>SPNIKIFSGSSHQDLSQKIADRLGLELGKVVTKKFSNQETCVEIGESVRGEDVYIVQSGCGEINDNLMELLIMINACKIASASRVTAVIPCFPYARQDKKDKVGESRAPISAKLVANMLSVAGADHIITMDLHASQIQGFFDIPVDNLYAEPAVLKWIRENISEWRNCTIVSPDAGGAKRVTSIADRLNVDFALIHKERKKANEVDRMVLVGDVKDRVAILVDDMADTCGTICHAADKLLSAGATRVYAILTHGIFSGPAISRINNACFEAVVVTNTIPQEDKMKHCSKIQVIDISMILAEAIRRTHNGESVSYLFSHVPL[18x]

Phosphoribosyl pyrophosphate synthetase (PRPS) stands as the first and rate-limiting enzyme in the purine biosynthesis pathway. It catalyzes the pyrophosphorylation of D-ribose-5-phosphate (R5P), obtained from the glucose pentose phosphate pathway (PPP), at the 1’ hydroxyl group position, yielding the catalytic product 5-phosphoribosyl-ɑ-1-pyrophosphate (PRPP). PRPP serves as an essential metabolic intermediate for purine biosynthesis via both de novo and salvage pathways, as well as for the synthesis of pyrimidines, amino acids (tryptophan and histidine), and co-factors (NAD+ and NADP+). Conversely, PRPS2 displays ~94% identity with PRPS1 and shares exactly the same biochemical reaction.

However, PRPS2 shares 94% amino acid identity with PRPS1, with three non-conserved residues (V103, G104, E105, referred to as 3AA hereinafter) located in the Loop2 region of PRPS2 as one of the major variations in their amino acid sequences, as they are absent in PRPS1. To elucidate the function of 3AA, we solved the crystal structure of a PRPS1 chimeric variant, PRPS1( + 3AA) in complex with R5P, ApCpp, and Cd2+ ion by co-crystallization, where 3AA was inserted into the corresponding position of the PRPS1 Loop2. The structure confirmed that the insertion of 3AA led to the flipping of Loop2 and the outward movement of the α12’ helix. Notably, a non-conserved PRPS1 residue, K153’ (Q156’ in PRPS2), stabilized the α12’ helix through a hydrogen bond with the C-terminal residue L321’, which was well-observed in the PRPS1( + 3AA) structure. Meanwhile, the deletion of the α12’ helix from PRPS1 or PRPS2 abolished their enzymatic activity. These results suggest that the four non-conserved residues of PRPS (3AA and Q156’/K153’) are essential for the conformational regulation of the C-terminal α12’ helix and the subsequent enzymatic catalysis. Further kinetic analysis of PRPS chimeric variants (PRPS1 with 3AA insertion and K153Q mutation, PRPS1( + 3AA/K153Q); PRPS2 with 3AA deletion and Q156K mutation, PRPS2(-3AA/Q156A), hereinafter) exhibited switched enzymatic activities, where PRPS1( + 3AA/K153Q) displayed ~2-fold or 16-fold lower kinetic efficiency in R5P or ATP, respectively, compared to PRPS2(-3AA/Q156A). In contrast, 3AA in PRPS2 sterically blocked GDP binding at the allosteric site, abolishing the feedback inhibition response of PRPS2. These findings were further confirmed by feedback inhibition assays on chimeric variants of PRPS1( + 3AA/K153Q) and PRPS2(-3AA/Q156K), which exhibited switched GDP feedback inhibition responses. Conversely, the ectopic expression of PRPS1( + 3AA/K153Q) mirrored PRPS2 phenotypes, displaying stronger growth and migratory abilities than PRPS1.>MASGMIVTDAGADQPIVFVNRAFSTITGYAPNEVLGRNARFLQGPQTDAATVARLREAIAAARPIQERILNYRKDGQPFW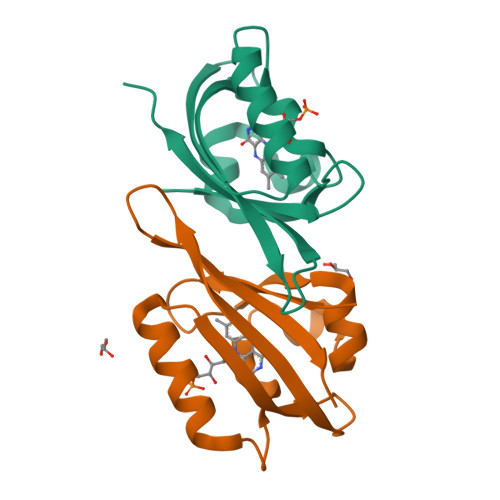NQLSISPVRDETGNVVAFVGVHTDVTAHHHHHH[2x]> MKREAIHNFFVANQIIKSTA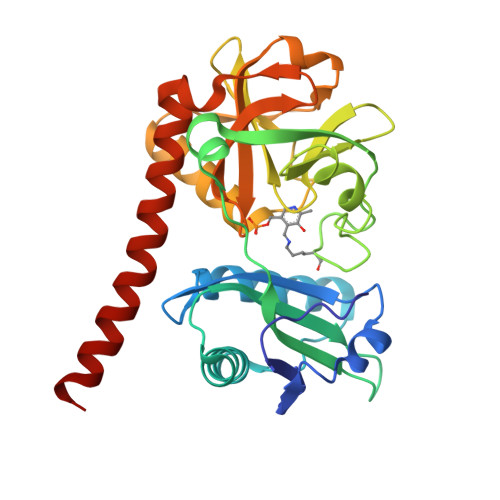DMAIFDKVPATAIYEVMQVRQGIPLFFEAHLERFVMSASLVGTRIPKKEAEILHNIADLVEKNKCDHGNVKLVSALMNEKEIFLAYFIPAEFLDSKARLEGVHTILFSGERICPNIKTIKGSFREQVKAVRESSNAYEALLVNESGHITEGSRSNVFFMGKDNKLYTSPAGSVLKGVTRTHVMQICSRLGLEVLEKTVHTRNLADIQGAFITGTTVDVTPVRSIGNTQLDSPNIPLIRKIVAEYEKKIAGYVSKRLKRARKVYVND>GSSGEGQKDLRLGELLLQKGWISREALEEALVEQEKTGDLLGRILVRKGLPEEALYRALAEQKGLEFLESTEGIVPDPSAALLLLRSDALRYGAVPIGFQNGEVEVVLSDPRHKEAVAQLLNRPARFYLALPQAWEELFRRAYPQK[2x]

The traffic ATPase PilF from Thermus thermophilus is important for type IV pilus biogenesis, twitching motility, surface attachment, and natural DNA-uptake and contains three consecutive homologous GPSII domains. The N-terminal part of PilF harbors a remarkable arrangement of three successive general secretory pathway II (GSPII) domains (GSPII-A to GSPII-C) with high sequence similarity to each other. Interestingly, we find that PilF binds only two molecules of c-di-GMP with different affinities and that the c-di-GMP–binding activities can be attributed to the GSPII-B and GSPII-C domains. Remarkably, the GSPII-B domain binds c-di-GMP with a KD of only 6 nM and thus with an affinity ∼ 83fold higher than MshEN.

Initially, we introduced arginine residues at these positions to reestablish an MshEN-like binding mode. We found a 25-fold higher KD value of 150 ± 7 nM for K167R compared to the WT (6 nM) and a 4-fold higher KD value of 23 ± 2 nM for L196R. The PilF159-302 K167R variant crystallized well and diffracted up to 1.8 Å with the macromolecular chain being traceable from residue 165 to 301 without interruption. The structure of chain A showed that in this mutant R167 is indeed involved in a cation-π-stacking interaction with the GMP1 guanine base. However, only partial electron density is observed for the side chain of R167 and the neighboring E170 in chain B of the crystal structure and there the R167 side chain guanidine group appears to be oriented towards a phosphate group of the ligand. Thus, the R167 stacking interaction with the guanine base of the ligand seems to be more dynamic and less energetically favorable than the equivalent interaction in the WT. In comparison to MshEN (chain A), the arginine side chain in chain A is positioned more towards the center of the guanine base. This is most likely due to the presence of E170, which positions R167 by forming simultaneous hydrogen bonds with its backbone amide and the guanidinium group of its side chain. The loss of binding affinity for PilF159-302 K167R in combination with the presence of a more dynamic cation-π-stacking interaction of R167 on the guanine base of GMP1 indicate that a lysine side chain at this position is beneficial for c-di-GMP binding most likely due to the presence of more extensive hydrophobic interactions.> MILFRKFRVLILTVFLIACTMHIMIDLL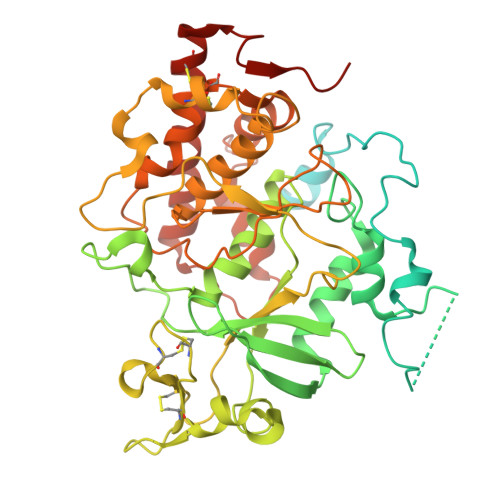PKLEKRAAGSSSSAGGGSGCSCAHTPGEEPRSWGKQRARAADPGWPNKHSLRLLQDFSNEPNSNLTSQSREKVTERAGSEKQGSGKRGLMREADSRQRRTDVRVSSVLQSLFEHPLYRTVLPDLTEEDTLFNLNAEIRLYPKAAGQQEWHNEGNVEEEEFSPPGEANSESYPNWLRFHIGINRYELYSRHNPVIAALLRDLLSQKISSVGMKSGGTQLKLIMSFQNYGQALFKPMKQTREQETPPDFFYFSDFERHNAEIAAFHLDRILDFRRVPPVAGRLVNMTREIRDVTRDKKLWRTFFVSPANNICFYGECSYYCSTEHALCGKPDQIEGSLAAFLPDLALAKRKTWRNPWRRSYHKRKKAEWEVDPDYCDEVKQTPPYDRGTRLLDIMDMTIFDFLMGNMDRHHYETFEKFGNDTFIIHLDNGRGFGKHSHDEMSILVPLTQCCRVKRSTYLRLQLLAKEEYKLSSLMEESLLQDRLVPVLIKPHLEALDRRLRLVLKVLSDCVEKDGFSAVVENDLDGQPSVHGGR> MAKLLQRVEITLRSFYIFNSTFGQVEGEEHKKVLFYHPNDIELNTKIKDVGLSEAIIRFTGTFTSEDDCQALHTQKTTQLFYQPEPGYWLVLVLNVPKEVRLKEGVEVADYRGAEISDRIYRAILRQCYQMFRFQNGCFSSCGSEEPNPDKRRELLCQKLLQFYDQHLTNLRDPAQCDIIDMLHSIQYLPLDKTLFLRAQNFGTLCETFPDIKESIMLYQ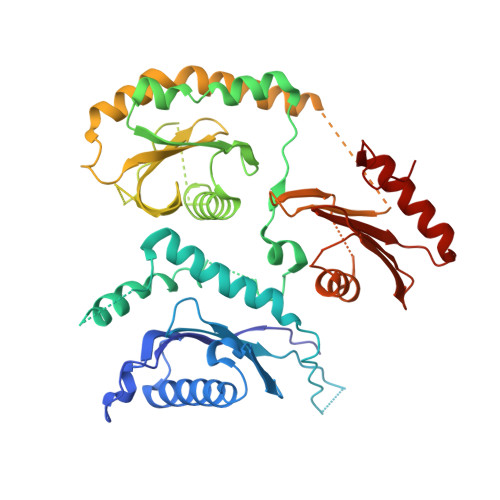EQVLCGGKLSPEDLHCVHSYVVQHVLKVEASSSTIAVSPSLKRSISECQVGGFVRSRQKVAGDEHDAVNEEDHPMKVYVTLDKEAKPYYLLIYRALHITLCLFLNADQVAPKQDLYDDLHAYMAPQLTSLARDISSELTKEAVGAAGQDNSSGNSETAPKYLFINEQSLQHHTNFQRHLPQGLPRNVLSIIADLANGSGKAEMESAPAEEVQVKTTNDYWIVKRRCNYRQYYVILCNSKATLLDVTQEARRIFEQELTDDVFFDK> MRDIVFVSPQLYLSSQEGWKSDSAKSGFIPIL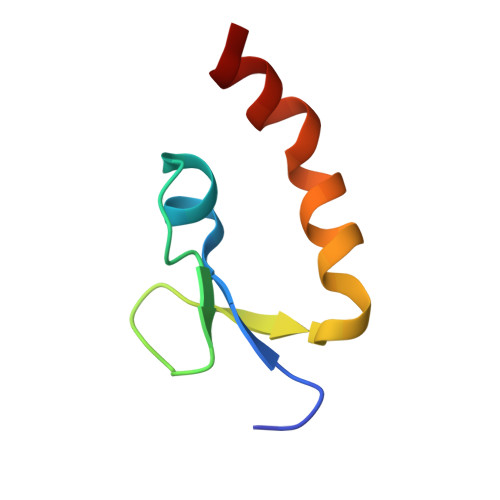KNDLQRFQDSLKHIVDARNS>[3x]SRNTPDRRQRAAGDAERTQSMRLQQKINDLKPYVRHARGPIKAYGQAALDRASGAATSVSFAELDATHLDAMVYIENQRNPGLNLKHFRDHYYLIQALQSDGPSAFRAIFPQTCPETGQTLK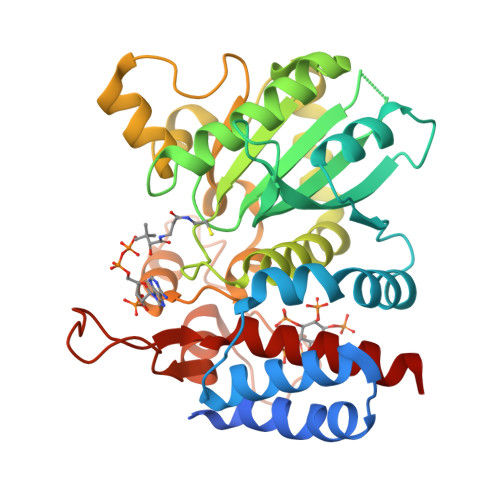HHVMADVRLHQGGAPTIIITEPAVIVGARYQQLQRHNLTLEDLSESGVPLSQVAIIETQAQKTSDDCVMYSLNYAIKAHKNAAQFDDIHHGLQHGTLSTESESRARTTLGALEASSSYSVMHEGAHAAFGADVLPVDFYKHGASLTQAYYLMKRPDGRMAGRVNSEGHSEAENLVQRNQAFRVKRRELLDDETPSNTQFSASIDGFRLQEIKRVLAAAQR>MAHHHHHHMQNYLHLLQDILDNGSDKTDRTGTGTRSLFGYQLRYDLSKGFPLVTTKKVHLKSIIYELLWFLKGDTNIKYLKDNGVSIWDEWADENGDLGPVYGAQWRSWRGADNKVVDQISEVIDQIKKNPDSRRLIVSAWNVAEIPNMA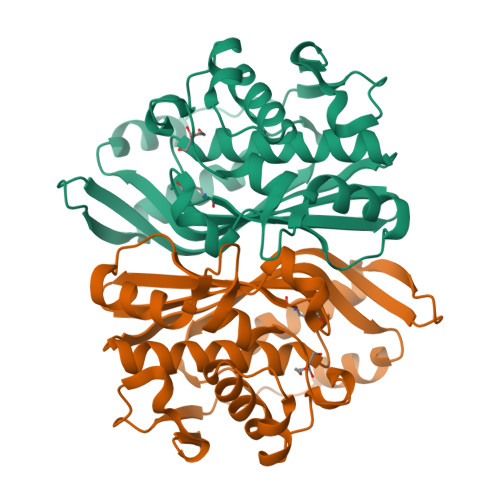LAPCHAMFQFYVADGKLSLQLYQRSADVFLGVPFNIASYALLLMMVAQVTGLQVGDYVHSFGDVHIYNNHFEQVNRQLSRDPKPLPVMKLNPDVKDIFDFKFEDFELLNYDPHPGIKAPVAI[3x]>[2x]MAHSSATAGPQADYSGEIAELYDLV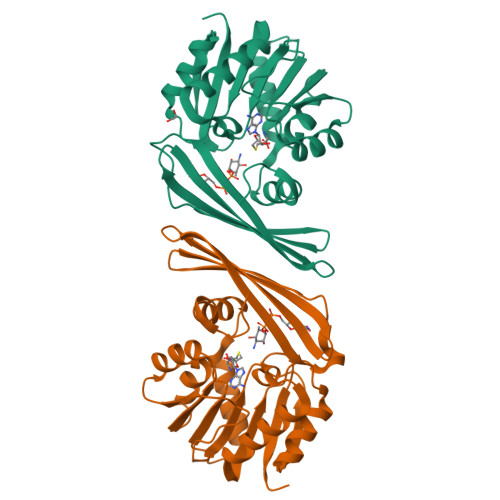HQGKGKDYHREAADLAALVRRHSPKAASLLDVACGTGMHLRHLADSFGTVEGLELSADMLAIARRRNPDAVLHHGDMRDFSLGRRFSAVTCMFSSIGHLAGQAELDAALERFAAHVLPDGVVVVEPWWFPENFTPGYVAAGTVEAGGTTVTRVSHSSREGEATRIEVHYLVAGPDRGITHHEESHRITLFTREQYERAFTAAGLSVEFMPGGPSGRGLFTGLPGAKGETRLEHHHHHH>[2x]MPVLEPTTQKFINALSASGGPAIYTLTPAEARDVLSGAQSGEIAKPAVDITDTTFAVGPTGATKVRIIRPQGNTDRLPVIVY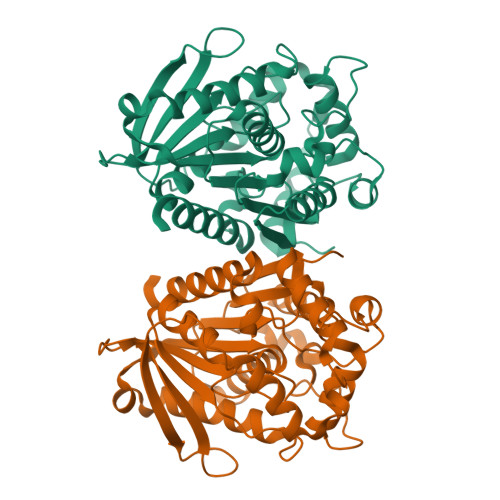FHGAGWVMGDTGTHDRLVRELSVRANAALVFVDYERSPEARYPVAIEQDYAVTKYVAEHSEQLNVDPTRLAIAGDSVGGNMTAVVSLLAQERGGPDITAQVLFYPVTDADFDNGSYTEFANGPWLTKPAMDWFWNQYLPEGIDRTDPKITPIHATSEQLSGQAPALVITAENDVLRDEGEAYARKLSQAGVDVTVTRYNGTIHDFVMLNVLADTPAAKGAIAQAGQYLHTALHGKHHHHHH THIOSULFATE | O3 S2 | 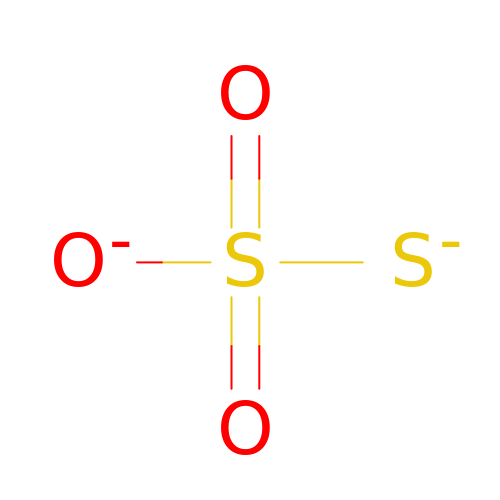DHCDFWKWKRSZHF-UHFFFAOYSA-L> MS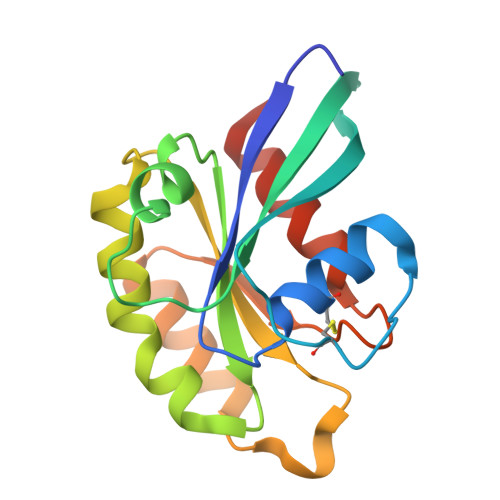YSYIFKYIIIGDMGVGKSCLLHQFTEKKFMADCPHTIGVEFGTRIIEVSGQKIKLQIWDTAGLERFRAVTRSYYRGAAGALMVYDITRRSTYNHLSSWLTDARNLTNPNTVIILIGNKADLEAQRDVTYEEAKQFAEENGLLFLEASAKTGENVEDAFLEAAKKIYQNIQDGS>[6x]MSTLSGPQYLGEGLKLMMRPGLRLFVLLPLSINLILFIGLIGFAINQFSHWVDWLMPSLPEWLSFLQFILWPLFVTLVLLIVFFTFTLIANLIAAPFNGFLAEKVEVVVRGTDDFPAFSWAELMAMVPRTIGRELRKLGYFLPRAIALFILSLIPGLNLIAAPLWLLFGVWMMAVQYIDYPADNHKLGWNEMLAWLRSKRWACMGFGGITYLVLLIPLVNLVAMPAAVAGAVLFWVREGGDQALVK

CysZ family members are 28–30 kDa bacterial inner-membrane proteins found exclusively in prokaryotes with no apparent homology to any of the established channel or transporter folds, and are scarcely studied in the literature. The CysZ protomer is an alpha-helical integral membrane protein with two long transmembrane (TM) helices (H2b and H3a) and two pairs of shorter helices (H4b-H5a and H7-H8) that insert only partially into the membrane (hemi-penetrating), forming a funnel or tripod-like shape within the membrane. The protein has an extra-membranous hydrophilic ‘head’, comprising an iris-like arrangement of the two short helices, H1 and H6, and kinked helices H3b, H4a, and H5b. Besides not resembling other transporter structures, CysZ mediates sulfate flux into cells or proteoliposomes without coupling to ion gradients, partner proteins, or exogenous energy sources such as ATP.

Third, we determined the structure of PdCysZ, which crystallized in multiple forms belonging to space groups P63, P4122 and P212121, revealing the same architecture and oligomeric assembly each time. We focused our analysis on the best of these (3.4 Å resolution in P63). The location of the selenium sites was obtained from a SeMet SAD data set, and the structure was solved by combining the resulting SAD phases with those from a molecular replacement solution obtained by positioning the PfCysZ model (75% sequence identity) onto SeMet fiducials in the initial electron density map. The refined structure of PdCysZ comprises an entire hexamer of near-perfect D3 symmetry. Antiparallel pairs of protomers arrange together as a trimer of dimers, with the three-fold axis oriented perpendicular to the plane of the putative membrane and three two-fold axes between dimers of the hexamer. Both the periplasmic and cytoplasmic faces of the hexamer are essentially identical by symmetry, resulting in a dual-topology assembly for PdCysZ. The hexamer has a triangular face of equal sides measuring approximately 75 Å, with the perpendicular span of about 65 Å. A surface electrostatic representation reveals a hydrophobic belt along the mid-section of the hexamer when viewed from its side, outlining the orientation of CysZ in the lipid bilayer. In the structure of PdCysZ, the entrance of the putative pore appears to be closed by the network of charge-interactions by conserved residues, R110, E106, N184, H185 and W235. Following this polar environment, the putative pathway widens even further leading into a large, primarily hydrophobic, internal cavity encapsulated by the TM helices of the PdCysZ hexamer, located in the plane of the lipid bilayer.> MPENVAPRSGATAGAAGGRGKGAYQDRDKPAQIRFSNISAAKAVADAIRTSLGPKGMDKMIQDGKGDVTITNDGATILKQMQVLHPAARMLVELSKAQDIEAGDGTTSVVIIAGSLLDSCTKLLQKGIHPTIISESFQKALEKGIEILTDM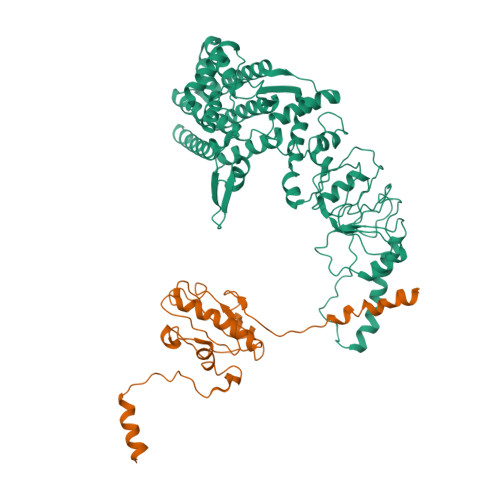SRPVELSDRETLLNSATTSLNSKVVSQYSSLLSPMSVNAVMKVIDPATATSVDLRDIKIVKKLGGTIDDCELVEGLVLTQKVSNSGITRVEKAKIGLIQFCLSAPKTDMDNQIVVSDYAQMDRVLREERAYILNLVKQIKKTGCNVLLIQKSILRDALSDLALHFLNKMKIMVIKDIEREDIEFICKTIGTKPVAHIDQFTADMLGSAELAEEVNLNGSGKLLKITGCASPGKTVTIVVRGSNKLVIEEAERSIHDALCVIRCLVKKRALIAGGGAPEIELALRLTEYSRTLSGMESYCVRAFADAMEVIPSTLAENAGLNPISTVTELRNRHAQGEKTAGINVRKGGISNILEELVVQPLLVSVSALTLATETVRSILKIDDVVNTR;> MQDPNADTEWNDILRKKGILPPKESLKELEEEAEEEQRILQQSVVKTYEDMTLEELEDHEDEFNEEDERAIEMYRRRRLAEWKATKLKNKFGEVLEISGKDYVQEVTKAGEGLWVILHLYKQGIPLCALINQHLSGLARKFPDVKFIKAISTTCIPNYPDRNLPTIFVYLEGDIKAQFIGPLVFGGMNLTRDELEWKLSESGAIMTDLEENPKKPIEDVLLSSVRRSVLMKRDSDSEGD LAEVULINIC ACID | C5 H8 O3 | 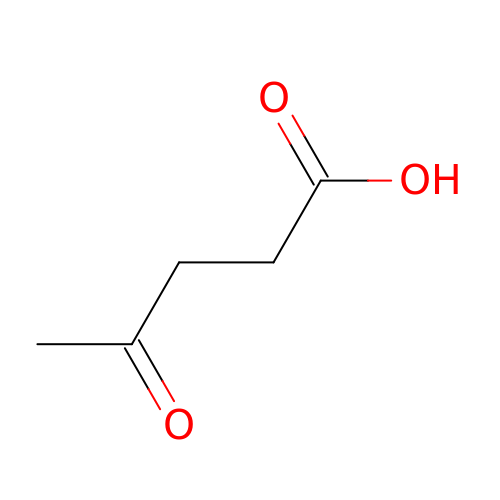JOOXCMJARBKPKM-UHFFFAOYSA-N3,5,7-trihydroxy-2-(3,4,5-trihydroxyphenyl)chromenium | 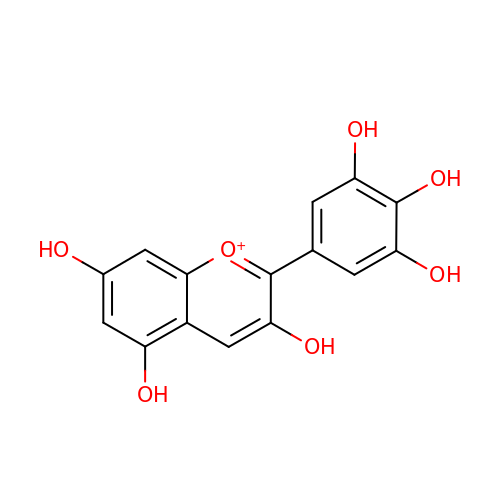C15 H11 O7 | JKHRCGUTYDNCLE-UHFFFAOYSA-O>[4x]V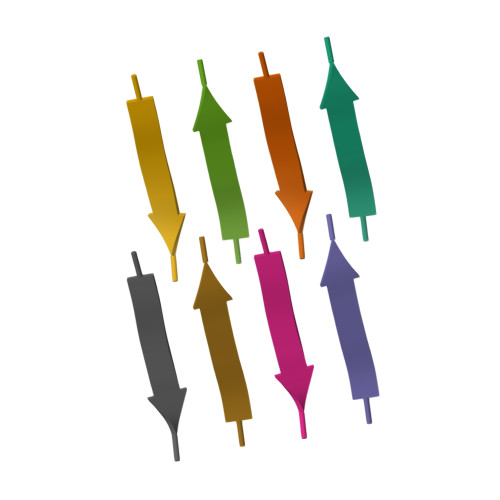EALYL>MAAGIVASRRLRDLLTRRLTGSNYPGLSISLRLTGSSAQEEASGVALGEAPDHSYESLRVTSAQKHVLHVQLNRPNKRNAMNKVFWREMVECFNKISRDADCRAVVISGAGKMFTAGIDLMDMASDILQPKGDDVARISWYLRDIITRYQETFNVIERCPKPVIAAVHGGCIGGGVDLVTACDIRYCAQDAFFQVKEVDVGLAADVGTLQRLPKVIGNQSLVNELAFTARKMMADEALGSGLVSRVFPDKEVMLDAALALAAEISSKSPVAVQSTKVNLLYSRDHSVAESLNYVASWNMSMLQTQDLVKSVQATTENKELKTVTFSKL[6x]

Here we report the use of single particle cryo-EM to identify multiple proteins from three enriched heterogeneous fractions prepared from human liver mitochondrial lysate. Using this approach, we were able to simultaneously identify and solve cryo-EM structures of nine different human mitochondrial enzymes: short chain acyl-CoA dehydrogenase (SCAD), medium chain acyl-CoA dehydrogenase (MCAD), isovaleryl-CoA dehydrogenase (IVD), delta (3, 5)-delta dienoyl-CoA isomerase (ECH1), aspartate aminotransferase (GOT2), glutamate dehydrogenase (GLUD1), mitochondrial superoxide dismutase 2 (SOD2), catalase (CAT), and mitochondrial aldehyde dehydrogenase (ALDH2). Functionally, the three acyl-CoA dehydrogenases—SCAD, MCAD and IVD—are involved in beta oxidation and amino acid catabolism. Finally, SOD2, CAT, and ALDH2 are all involved in clearing toxic byproducts of oxidative respiration.

The first enzyme in this pathway, ECH1, shifts double bonds from positions 3 and 5 to positions 2 and 4, isomerizing 3,5-dienoyl CoA to 2,4-dienoyl CoA. A total of 8862 single particle cryo-EM projections were collected for this structure. From these projections, we constructed a high-resolution cryo-EM map of 2.96 Å and identified this protein as the ECH1 isomerase. The overall structure is a hexamer made up of a pair of trimers. Each monomer has two domains: an N-terminal catalytic domain and a C-terminal α-helical domain. Similar to other members of the isomerase family, the N-terminal domain is a spiral of four turns. Each turn is made up of two β strands followed by one or two α helices. The C-terminal domain is made up of a core of four α helices that interact with the other two subunits to form the trimerization domain. The trimer–trimer interface is formed by the interaction of the α-helix from the second turn in the catalytic domain interacting with the trimerization domain. We did not observe a bound ligand in our cryo-EM structure but a previously solved rat crystal structure identified equivalent catalytic residues as I118, D177, E197, and D205.> EFSMKSVKGLLFIIASFILTLLTWMNTSPQFMIPGLALTSLSLTFILATRLPLLESWFHSLEKVYTVHKFTAFLSIILLIFHNFSMGGLWGSRLAAQFGNLAIYIFASIILVAYLGKYIQYEAWRWIHRLVYLAYILGLFHIYMIMGNRLLTFNLLSFLVGSYALLGLLAGFYIIFLYQKISFPYLGKITHLKRLNHDTREIQIHLSRPFNYQSGQFAFLKIFQEGFESAPHPFSISGGHGQTLYFTVKTSGDHTKNIYDNLQAGSKVTLDRAYGHMIIEEGRENQVWIAGGIGITPFISYIREHPILDKQVHFYYSFRGDENAVYLDLLRNYAQKNPNFELHLIDSTKDGYLNFEQKEVPEHATVYMCGPISMMKALAKQIKKQNPKTELIYEGAKFK

Evolutionarily distant proteins with the NOX catalytic core have been found in bacteria, including Streptococcus pneumoniae NOX (SpNOX), which is proposed as a model for studying NOXs because of its high activity and stability in detergent micelles. NOXs belong to the ferric reductase transmembrane component-like domain (FRD) superfamily and are composed of a catalytic core with two conserved domains: a domain with six transmembrane helices (TM domain) coordinating two hemes by four conserved histidine residues and a C-terminal cytosolic dehydrogenase domain (DH domain) containing the flavin adenine dinucleotide (FAD)-binding and NADPH-binding sites. The DH domain catalyzes a hydride transfer to FAD, which subsequently transfers electrons stepwise to the two transmembrane hemes. The structure of SpNOX corresponds to the canonical NOX structure, with an N-terminal TM domain that coordinates two hemes and a C-terminal DH domain bound to FAD.

We present here cryo-electron microscopy structures of substrate-free and nicotinamide adenine dinucleotide (NADH)-bound SpNOX and of NADPH-bound wild-type and F397A SpNOX under turnover conditions. These high-resolution structures provide insights into the electron-transfer pathway and reveal a hydride-transfer mechanism regulated by the displacement of F397. As for other members of the FNR superfamily, a transient displacement of a C-terminal aromatic residue is necessary to perform hydride transfer. Here, we analyzed the steady-state kinetics of an F397A SpNOX mutant. Similarly to nNOS, we did not observe a large effect on the KM, which suggests that F397 does not have a major role in the control of NADPH-binding affinity in SpNOX. As for the F397S SpNOX mutant described in the previous study, we observed a moderate increase in kcat, which could be explained by the elimination of the F397 displacement step. These data are supported by further analysis of a cryo-EM structure of the F397A mutant bound to NADPH under turnover conditions at 2.64-Å resolution. Density can be observed for the bound substrate but, compared to the other substrate-bound structures described here, the nicotinamide is closer to the isoalloxazine ring. The absence of the large side chain of F397 allows NADPH to take up a productive conformation in SpNOX for pea FNR Y308 mutants. In this conformation, the nicotinamide ring does not lie parallel to the isoalloxazine ring but at a ~26° angle.In this study, we have characterized ZitRMG, a metallo-regulator of the MarR superfamily. In L. lactis subspecies cremoris strain MG1363, we have showed that ZitR repressor controls an emergency response to Zn(II) starvation, allowing Zn(II) uptake under extreme conditions, while impeding it in a wide concentration range, from repletion to toxicity. In solution, ZitRMG has been shown to be a stable dimer able to bind, as expected, both Zn(II) and double-stranded DNA fragments bearing the palindromic TTAACYRGTTAA recognition sequence. ZitRMG protein is folded as a triangular-shaped homo-dimer with a two-fold pseudo-symmetric axis, a typical topology for a MarR superfamily member.

The structure of ZitRMG holo-form was first determined at low resolution by single anomalous wavelength dispersion (SAD) and then, after crystal improvement by molecular replacement, at 2.8 Å resolution. The asymmetric unit (ASU) contained 8 ZitRMG molecules, and 16 Zn(II) atoms. ZitRMG molecules formed four dimers (AB, CD, EF and GH), all binding four Zn(II) atoms in total (two per protomer). In AB, both protomers have almost the same conformation and superimpose to each other with all 1144 atoms-RMSD of 0.34 Å. Each protomer is arranged from the N- to the C-terminus as follows: α1 (residues 3–17), α2 (residues 37–48), α3 (residues 53–60), α4 (residues 64–77), β1 (residues 80–83), β2 (residues 93–96), α5 (residues 100–124) and α6 (residues 127–144), in good agreement with our above-mentioned CD results, and as expected for a typical MarR superfamily member. In ZitRMG dimerization interface, the N-terminal α1 helix (protomer A), which is stacking between α5'-α6' helices, interacts with α1’, its counterpart in protomer B, and the same holds true for the C-terminal α6 and α6' helices. In ZitRMG like in E. coli MarR, streptococcal AdcR proteins and ZitRIL, the DNA-binding domain is folded as a wHTH domain made of a helix region (formed by α2, α3 and α4 helices) and a β strand region (β1 and β2 strands). The two metal binding sites of ZitRMG protein, like those of ZitRIL and AdcRSpne, are located at opposite sides of the dimer and two Zn(II) ions are bound per protomer. Glu23ZitR, His41ZitR and His111ZitR are moderately exposed, while His107ZitR is buried. Zn(II) is clearly coordinated by Oε1-Glu23ZitR, Nδ1-His41ZitR, Nε2-His107ZitR and Nε2-His111ZitR, although a supplementary coordination involving a second atom of the first ligand (Oε2) has also been proposed in AdcRSpne (see below). The three Zn(II) ligands in ZitRMG site 2: SH-Cys29ZitR, Oε1-Glu40ZitR (a buried residue), and Oε1-Glu106ZitR, are the same as in ZitRIL and AdcRSpne. Interestingly, ZitRMG is shown here to better align to the DNA-bound form of any MarR protein than to its DNA-free counterpart, suggesting that holo-ZitRMG dimer could be folded in a DNA-binding prone conformation.

>ALRNQIEQFLGAIMQFAENKHEILLGECESNVKLTSTQEHILMILAAEVSTNARIAEQLKISPAAVTKALKKLQEQELIKSSRATNDERVVLWSLTEKAIPVAKEHAAHHEKTLSTYQELGDKFTDEEQKVISQFLSVLTEEFR[8x]~{N}5-cyclopropyl-~{N}3-methyl-2-oxidanylidene-1-[(1~{R})-1-phenylethyl]pyridine-3,5-dicarboxamide | C19 H21 N3 O3 | 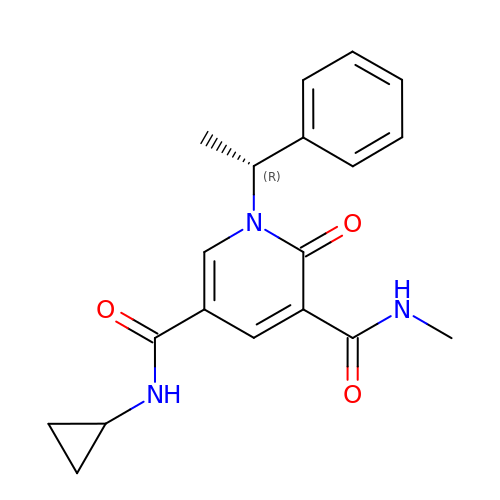AYQUCQJYWKQBRS-GFCCVEGCSA-N The enzyme SalBIII from the salinomycin biosynthetic pathway resembles other polyether epoxide hydrolases/cyclases of the MonB family, but SalBIII plays no role in the conventional cascade of ring opening/closing. Using this metabolite in vitro as a substrate analogue, SalBIII has been shown to form pyran ring A. We have determined the X-ray crystal structure of SalBIII, and structure-guided mutagenesis of putative active-site residues has identified Asp38 and Asp104 as an essential catalytic dyad. The demonstrated pyran synthase activity of SalBIII further extends the impressive catalytic versatility of α+β barrel fold proteins.

To provide a structural framework for understanding the activity of SalBIII, we have solved the X-ray crystal structure of SalBIII at 1.8 Å resolution. Phases were determined by molecular replacement. There are two protomers in the asymmetric unit, consistent with the fact that SalBIII is a homodimer in solution. Each subunit adopts the cone-shaped α+β barrel fold first recognized in the structure of scytalone dehydratase[10a] in which three or four α-helices pack against the concave side of a curved five- or six-stranded mixed β-pleated sheet, creating a largely hydrophobic active site cavity, closed at one end. The most similar 3D structures to that of SalBIII are those of the MonB-type epoxide hydrolases, but sequence alignment shows that in SalBIII one of the two catalytic residues (Asp38 and Glu65 in Lsd19/LasB N-terminal domain) is missing, and overall its sequence diverges significantly from other members of this family. Using the crystal structure of SalBIII as a guide, eight residues were identified as contributing to its active site: Tyr14, Asp38, Arg45, Tyr54, Asn58, Ile65, Asp104, and Trp121. In contrast, alteration of either Asp38 or Asp104 (to either Ala or Asn) gave wholly inactive mutants. These residues are suitably placed in the active site to operate as a catalytic dyad, to accomplish both dehydration and oxa-conjugate addition. Superimposition of the modeled active site structure of Cyc11 and that of Lsd19/LasB C-terminal domain[10e] onto the active site of SalBIII shows that they occupy exactly equivalent positions.

>MQDEQKRKEIVAEYFRKVNEGDVDAIVEMFTENATIEDPVGKDVREGRAAQREYFNSNVTAEVTIEPGHLSAGQDGKSVAVALAAEMTNILDPNRTRVKINAVDVFTLTPEGKIDSMRVFWGMTDIGVWNSSSVDKLAAALEHHHHHH[2x]~{N}-[5-[3-[[(4-hydroxyphenyl)amino]-bis(oxidanyl)-$l^{4}-sulfanyl]-4-methoxy-phenyl]-4-methyl-1,3-thiazol-2-yl]cyclopentanecarboxamide 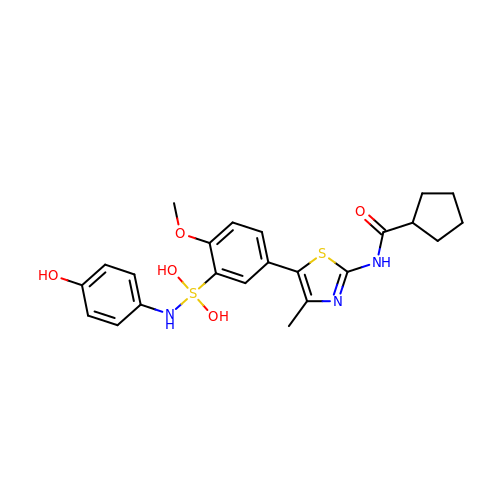| C23 H27 N3 O5 S2 | CBCKCOMPEQUVAG-UHFFFAOYSA-N>[4x]HTIFSSLEVNGVNQGLGEGVRVPTYNGPIEDVTSASIACNGSPNTVASTSKVITVQAGTNVTAIWRYMLSTTGDSPADVMDSS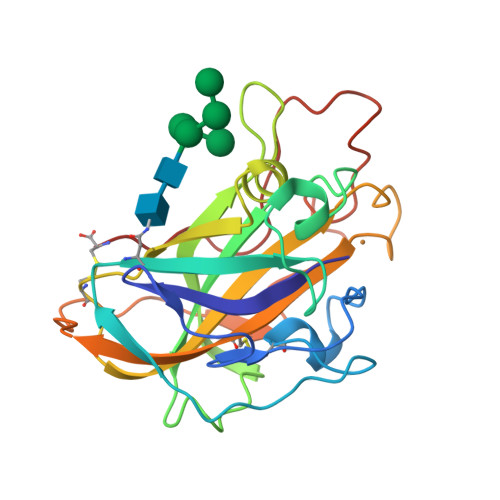HKGPTIAYLKKVDNAATASGVGNGWFKIQQDGMDSSGVWGTERVINGKGRHSIKIPECIAPGQYLLRAEMIALHAASNYPGAQFYMECAQLNVVGGTGAKTPSTVSFPGAYSGSDPGVKISIYWPPVTSYTVPGPSVFTC>HMQKVEVFRIPTASPDDISGLATLIDSGKINPAEIVAILGKTEGNGCVNDFTRGFATQSLAMYLAEKLGISREEVVKKVAFIMSGGTEGVMTPHITVFVRKDVAAPAAPGKRLAVGVAFTRDFLPEELGRMEQVNEVARAVKEAMKDAQIDDPRDVHFVQIKCPLLTAERIEDAKRRGKDVVVNDTYKSMAYSRGASALGVALALGEISADKISNEAICHDWNLYSSVASTSAGVELLNDEIIVVGNSTNSASDLVIGHSVMKDAIDADAVRAALKDAGIRSDDEMDRIVNVLAKAEAASSGTVRGRRNTMLDDSDINHTRSARAVVNAVIASVVGDPMVYVSGGAEHQGPDGGGPIAVIARV[4x]

The use of cyanuric acid hydrolase to solve this societal problem is being explored and the best candidate for this biotechnological application is the thermostable enzyme from Moorella thermoacetica. Consistent with the “Toblerone fold” observed for these enzymes[8–10], the RMCAH monomer is composed of three concatenated, highly divergent, but structurally homologous domains, which endows the enzyme monomer an internal pseudo-three-fold symmetry (Domains 1, 2). As observed for AtzD and ACAH, the active site of RMCAH lies on the pseudo-three-fold axis within each monomer and is formed by similar sets of residues from all three domains. As observed for ACAH and AtzD, each of the three serine γO atoms is in close proximity to a lysine residue (Lys40, Lys161 and Lys299), generating three pairs of Ser-Lys dyads each from one of the three isostructural domains from the same monomer.

By soaking the APO RMCAH crystal with the cyanuric acid analog and a competitive inhibitor barbiturate (BAR), we obtained a BAR-bound structure with all four monomers in the closed conformation. However, the significantly improved resolution, along with structures with other ligands reported in this study, enables a more thorough examination of the complex as well as comparative analysis. Both planar and non-planar BAR were used in the refinement, and the planar BAR fit in the electron density better. Even though the BAR electron density shows nearly three-fold symmetry, the bound BAR in the active site is likely orientated in a specific configuration based on its positioning relative to the surrounding protein residues. At A’ and B’ positions, the distance between a ring nitrogen atom of BAR and the backbone carbonyl oxygen atom of Gly84 and Ala232 from RMCAH are 2.8 and 3.0 Å, respectively, while at the C’ position, the distance between the α-carbon atom of BAR and Gly348 is 3.2 Å. Viewed from top of BAR along its pseudo three-fold axis, Ser83 and Ser347 γOs are both exterior to the ring, while Ser231 γO is directly above the BAR ring and points to the mid-point of BAR carbon atoms of carbonyl group at B and C. Each carbonyl oxygen atom of the inhibitor at the sites A, B, and C forms hydrogen-bonding interactions with a main chain amide nitrogen atom and an arginine side chain. The present RMCAH/BAR structure refined at 1.88 Å resolution shows that the αBD/αFL angles (110° and 5°) and the distance (3.4 Å) between the Ser231 γO and a substrate carbonyl group are well within favorable ranges for initializing the nucleophilic addition reaction, in contrast to unfavorable parameters for the other serine residues (Ser83 80°/35°/3.6Å, Ser347 45°/65°/3.6Å).> SVLQVLHIPDERLRKVAKPVEEVNAEIQRIVDDMFETMYAEEGIGLAATQVDIHQRIIVIDVSENRDERLVLINPELLEKSGETGIEEGCLSIPEQRALVPRAEKVKIRALDRD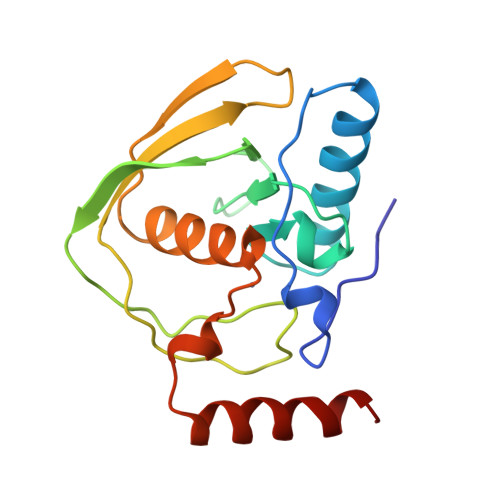GKPFELEADGLLAICIQHEMDHLVGKLFMDYLSPLKQQRIRQKVEKLDRL> LSEEQQHIIAILLDAH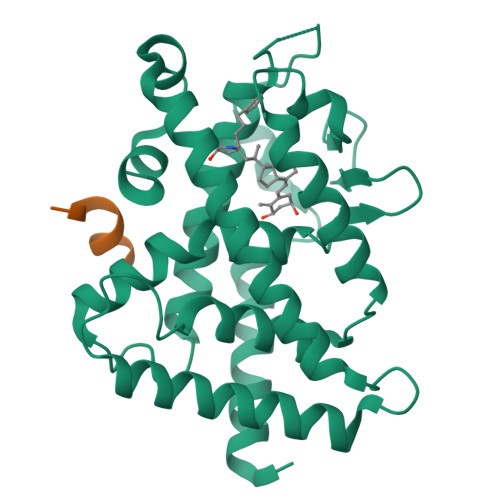HKTYDPTYADFRDFRPPVRMDGSTGSVTLDLSPLSMLPHLADLVSYSIQKVIGFAKMIPGFRDLTSDDQIVLLKSSAIEVIMLRSNQSFTMDDMSWDCGSQDYKYDVTDVSKAGHTLELIEPLIKFQVGLKKLNLHEEEHVLLMAICIVSPDRPGVQDAKLVEAIQDRLSNTLQTYIRCRHPPPGSHQLYAKMIQKLADLRSLNEEHSKQYRSLSFQPENSMKLTPLVLEVFG;> NHPMLMNLL> SKEGSVAPKERINIKYIPATGDAQAEVELPLKTLVVGDFKGHAEQTPLEERATVTVDKNNFEAVM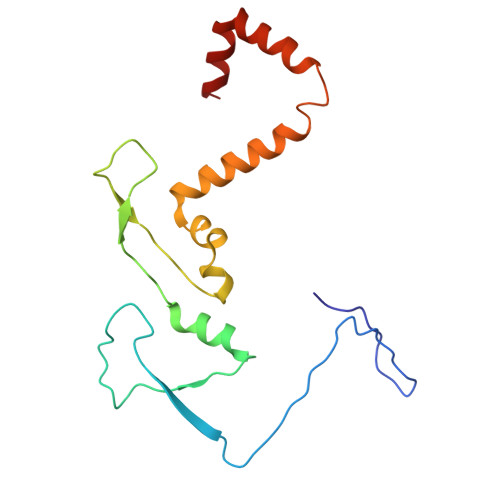RESELKITATVKNKLTDDENAELPVELNFKSLADFAPDAVASQVPELKKLIELREALVALKGPLGNIPAFRERLQSLLNSEESREKLLAE TOBRAMYCIN | C18 H37 N5 O9 | 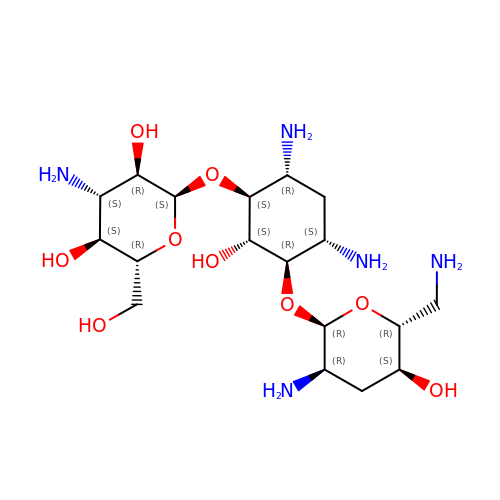NLVFBUXFDBBNBW-PBSUHMDJSA-N>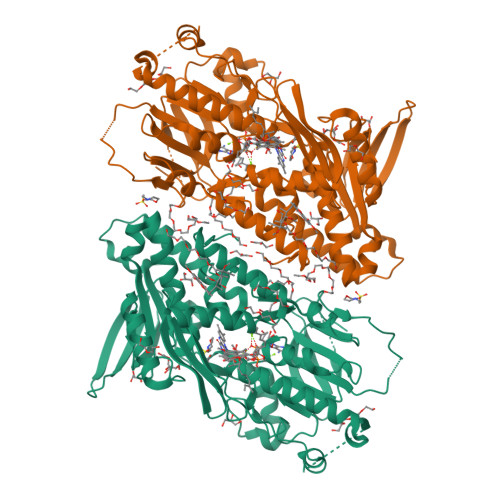 VENSGAGPTSFKTMKVIDPQHSDKPNVLILGSGWGAISFLKHIDTKKYNVSIISPRSYFLFTPLLPSAPVGTVDEKSIIEPIVNFALKKKGNVTYYEAEATSINPDRNTVTIKSLSAVSQLYQPENHLGLHQAEPAEIKYDYLISAVGAEPNTFGIPGVTDYGHFLKEIPNSLEIRRTFAANLEKANLLPKGDPERRRLLSIVVVGGGPTGVEAAGELQDYVHQDLRKFLPALAEEVQIHLVEALPIVLNMFEKKLSSYAQSHLENTSIKVHLRTAVAKVEEKQLLAKTKHEDGKITEETIPYGTLIWATGNKARPVITDLFKKIPEQNSSKRGLAVNDFLQVKGSNNIFAIGDNAFAGLPPTAQVAHQEAEYLAKNFDKMAQIPNFQKNLSSRKDKIDLLFEENNFKPFKYNDLGALAYLGSERAIATIRSGKRTFYTGGGLMTFYLWRILYLSMILSARSRLKVFFDWIKLAFFKRDFFKGL>[2x]SGHGMEENGMKSKILIFGGTGYIGNHMVKGSLKLGHPTYVFTRPNSSKTTLLDEFQSLGAIIVKGELDEHEKLVELMKKVDVVISALAFPQILDQFKILEAIKVAGNIKRFLPSDFGVEEDRINALPPFEALIERKRMIRRAIEEANIPYTYVSANCFASYFINYLLR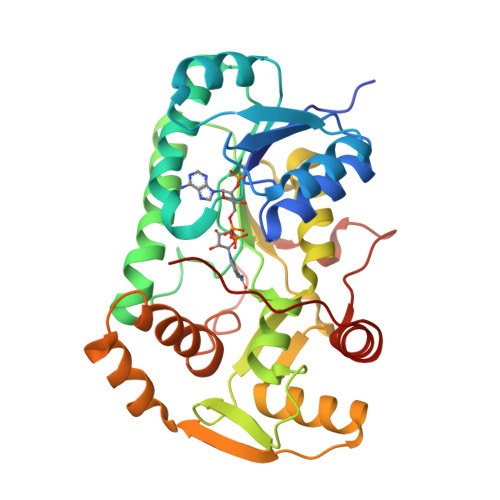PYDPKDEITVYGTGEAKFAMNYEQDIGLYTIKVATDPRALNRVVIYRPSTNIITQLELISRWEKKIGKKFKKIHVPEEEIVALTKELPEPENIPIAILHCLFIDGATMSYDFKENDVEASTLYPELKFTTIDELLDIFVHDPPPPASAAF methyl (2S)-2-[[2-methyl-3-oxidanyl-5-(phosphonooxymethyl)pyridin-4-yl]methylamino]-4-methylsulfanyl-butanoate 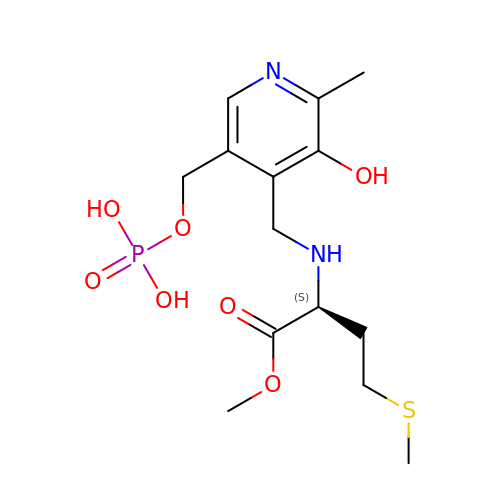| C14 H23 N2 O7 P S | XFBSUAILPATRCO-LBPRGKRZSA-N>SDKPVAHVVANHQVEEQLEWLSQRANALLANGMDLKDNQLVVPADGLYLVYSQVLFKGQGCPDYVLLTHTVSRFAISYQEKVNLLSAVK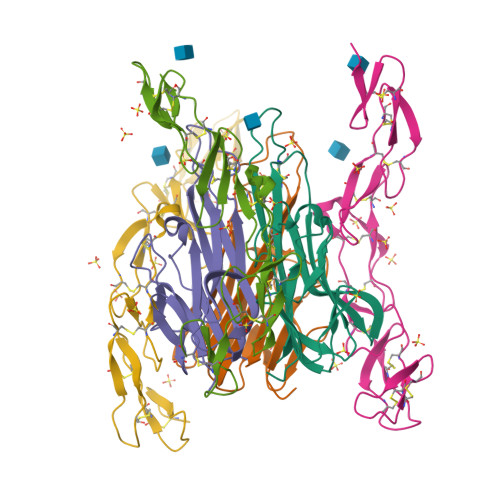SPCPKDTPEGAELKPWYEPIYLGGVFQLEKGDQLSAEVNLPKYLDFAESGQVYFGVIAL[3x];>GSVCPQGKYIHPQDNSICCTKCHKGTYLYNDCPGPGQDTDCRECESGSFTASENHLRHCLSCSKCRKEMGQVEISSCTVDRDTVCGCRKNQYRHYWSENLFQCFNCSLCLNGTVHLSCQEKQNTVCTCHAGFFLRENECVSSSN[3x]> MFARAFSRFASLAAPAPQRGWNAFVLPSRHFATAAGGANPFKNQLLLTLSSPSEAI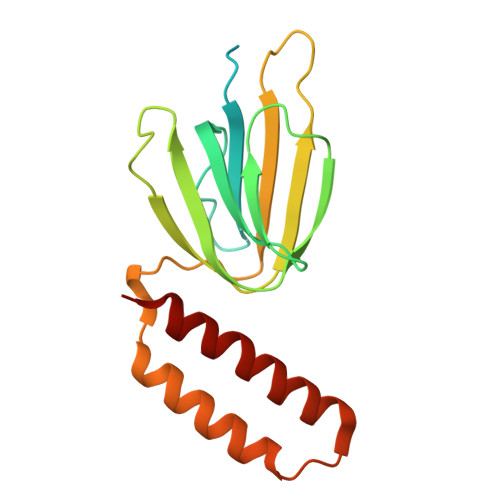YVRTPVRSVTVPGSEGAMTMTNGHSQTVARLKAGEIIVRKGETGDEVERFFLSDGFVLFKSPEDDSGCCTAEVLGVEVVPVSMLDKESAATALQELLQQGAGATDEWTKARTLLGQELLSSVIRAAP> GARDDEYDYLFKVVLIGDSGVGKSNLLSRFTRNEFNLE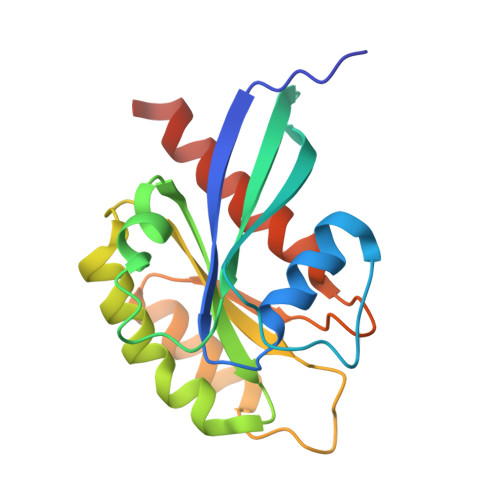SKSTIGVEFATRSIQVDGKTIKAQIWDTAGLERYRAITSAYYRGAVGALLVYDIAKHLTYENVERWLKELRDHADSNIVIMLVGNKSDLRHLRAVPTDEARAFAEKNGLSFIETSALDSTNVEAAFQTILTEIYRIVSQKQMSDRRE>[8x]DKLTLWTTLDPSPNCRIDVDKDSKLTLVLTKCGSQILANVSLLVVKGRFQNLNYKTNPNLPKTFTIKLLFDENGILKDSSNLDKNYWNYRNGNSILAEQYKNAVGFMPNLAAYPKSTTTQSKLYARNTIFGNIYLDSQAYNPVVIKITFNQEADSAYSITLNYSWGKDYENIPFDSTSFTFSYIAQE

Each protein forms key interactions to promote cell infection, with the terminal domain of the fiber, the fiber knob protein, interacting with the viruses’ primary cell entry receptor. The adenovirus fiber knob protein is known to have a highly conserved trimeric structure. Sialic acid (SA) usage has been proposed as a cell infection mechanism for EKC causing HAdV-D. Here we highlight an important role for SA engagement by many HAdV-D. We provide apo state crystal structures of 7 previously undetermined HAdV-D fiber-knob proteins, and structures of HAdV-D25, D29, D30 and D53 fiber-knob proteins in complex with SA. Our findings demonstrate a conserved binding site for sialic acid, common across the species D adenoviruses, therefore suggesting that, along with CAR, the receptor can be used to initiate cell entry.

HAdV-D15, D24 and D32 were crystallised in only their apo states, whereas HAdV-D25, D29, D30 and D53 crystals were also soaked with sialic acid. In this article we present seven novel structures of apo state fiber-knob proteins of species D adenoviruses. These provide a good basis from which to conduct structural analyses.>[2x]SMGALKCTFSAPSHSTSLLQGLATLRAQGQLLDVVLTINREAFPAHKVVLAACSDYFRAMFTGGMREASQDVIELKGVSARGLRHIIDFAYSAEVTLDLDCVQDVLGAAVFLQMLPVVELCE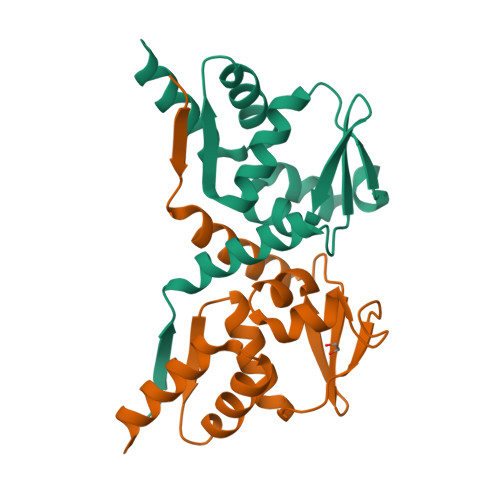EFLKAAMS> MLARRIVAKHVTKTTALAMLGTTIVLVILQVLFTYLGELSNLKADYSAWQAFLYVLWGAPRYLYEILPISALIGAILGLGTLASNSELIVMRSVGISLWRIVGWVIRSALVLVLLSFALSEWVVPYTNERANSVKSHQSVAALGEVRGYWSREGQRFIYVDYANSQGQLKRIQVVDFDDNYRLKSVTNAEQGQFVKDGQWLLNHSQQMAIQGQGDAVLANAAKQPFSLALQPKYVHMVTIDPEDLSFSQLVSFMNYMREYSQVPKTYQLAFWKKVASPFALITLVLVACSFIFGPLRQQSMGFRLVIALFIGLGFY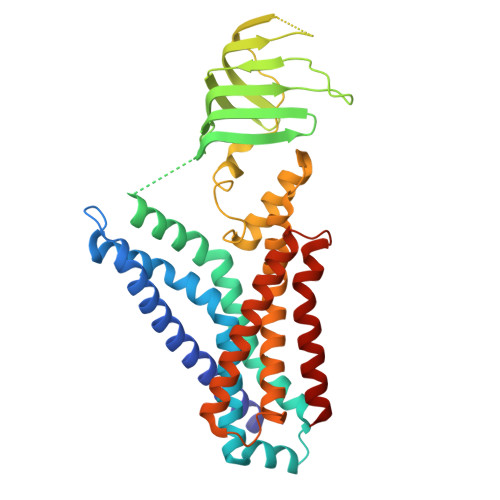YLQDFLGYASLVYNPSPAWFVLGPIVLMFVAGSYLLYRAR> MNQRPIQTATLSWNEQGTPVSEQFGDIYFSNEDGLEETHHVFLKGNGFPARFASHPQQSCIFAETGFGTGLNFLTLWRDFALFRQQSPNATLRRLHYISFEKYPLHVADLASAHARWPELASFAEQLRAQWPLPLAGCHRILLADGAITLDLWFGDVNTLLPTLDDSLNNQVDAWFLDGFAPAKNPDMWNEQLFNAMARMTRPGGTFSTFTAAGFVRRGLQQAGFNVTKVKGFGQKREMLTGTLPQQIHAPTAPWYHRPAATRCDDIAIIGGGIVSALTALALQRRGAVVTLYCADAQPAQGASGNRQGALYPLL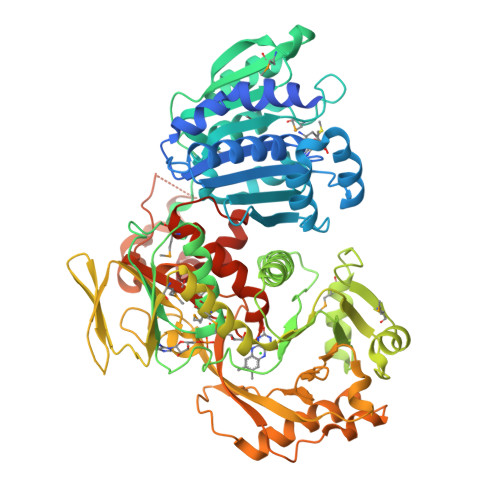NGKNDALETFFTSAFTFARRQYDQLLEQGIAFDHQWCGVSQLAFDDKSRGKIEKMLHTQWPVEFAEAMSREQLSELAGLDCAHDGIHYPAGGWLCPSDLTHALMMLAQQNGMTCHYQHELQRLKRIDSQWQLTFGQSQAAKHHATVILATGHRLPEWEQTHHLPLSAVRGQVSHIPTTPVLSQLQQVLCYDGYLTPVNPANQHHCIGASYQRGDIATDFRLTEQQENRERLLRCLPQVSWPQQVDVSDNQARCGVRCAIRDHLPMVGAVPDYAATLAQYQDLSRRIQHGGESEVNDIAVAPVWPELFMVGGLGSRGLCSAPLVAEILAAQMFGEPLPLDAKTLAALNPNRFWIRKLLKGRPVQTRSPATQESSR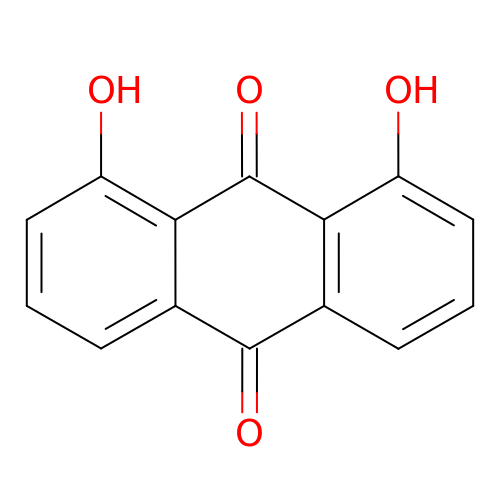1,8-dihydroxyanthracene-9,10-dione | C14 H8 O4 | QBPFLULOKWLNNW-UHFFFAOYSA-N> GAMREYKLVVLGSGGVGKSALTVQFVQGIFVEKYDPTIEDSYRKQVEVDAQQCMLEILDTAGTEQFTAMRDLYMKNGQGFALVYSITA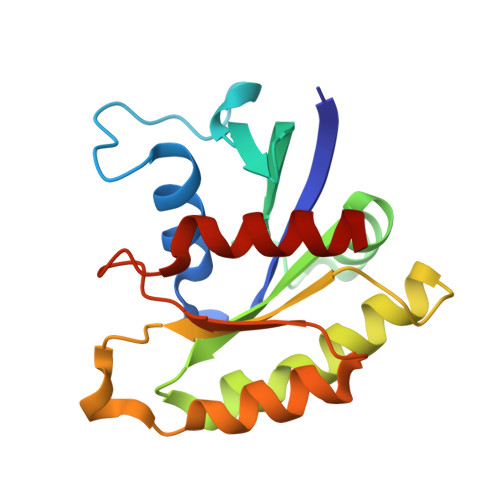QSTFNDLQDLREQILRVKDTDDVPMILVGNKCDLEDERVVGKEQGQNLARQWNNCAFLESSAKSKINVNEIFYDLVRQINR> RANDAPIVLLHGFTGWGREEMFGFKYWGGVRGDIEQWLNDNGYRTYTLAVGPLSSNWDRACEAYAQLVGGTVDYGAAHAAKHGHARFGRTYPGLLPELKRGGRIHIIAHSQGGQTARMLVSLLENGSQEEREYAKAHNVSLSPLFEGGHHFVLSVTTIATPHDGTTLVNMVDFTDRFFDLQKFVLKAAAVASNVPYTSQVYDFKLDQWGLRRQPGESFDQYFERLKRSPVWTSTDTARYDLSVPGAEKLNQWVKASPNTYYLSFATERTYRGALTGNYYPELGMNAFSAVVCAPFLGSYRNATLGIDDRWLENDGIVNAFSMNGPKRGSTDRIVPYDGTIKKGVWNDMG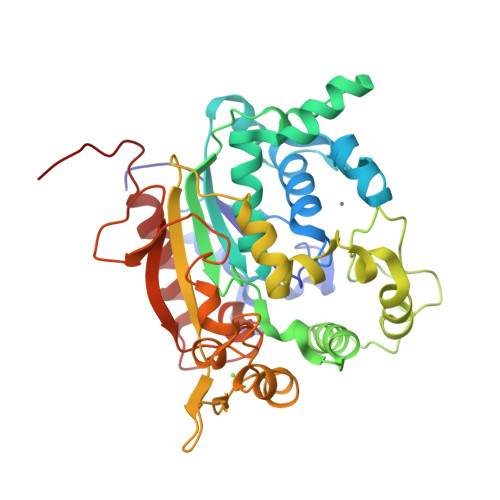TYNVDHLEVIGVDPNPLFDIRAFYLRLAEQLASLQPHHHHHH>GSMTNIPFIYQYEEKENERAAAGYGTFGYLITRIEETLYDQYGVFYELYASDDPNTEYWELLVEDVRSGSLEPEHVAYIFEKLEKKTFAYDEDEKEPDYTVHKSIRNSVYAYPEKGVAFARIPYFQDGSIMSFDCLFAVNDEKMRAFLEGVRPR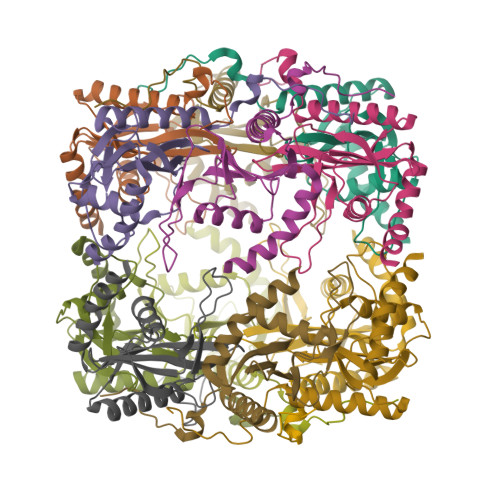LWEKSKR[12x]> MHHHHHHSSGRENLYFQGCCEHHKAMIAGLALLRNPELLLEIPLALLVVGLGGGSLPLFVHDHFPKSCIDAVEIDPSMLEVATQWFGFSQSDRMKVHIADGLDYIASLAGGGEARPCYDVIMFDVDSKDPTLGMSCPPPAFVEQSFLQKVKSILTPEGVFILNLVCRDLGLKDSVLAGLKAVFPLLYVRRIEGEVNEILFCQLHPEQKLATPELLETAQALE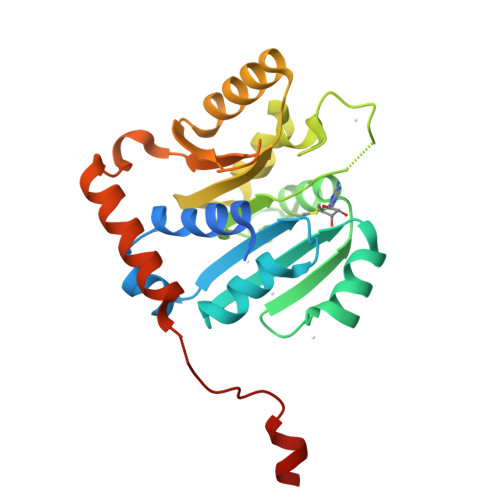RTLRKPGRGWDDTYVLSDMLKTVKIV>MAPKGTSLDEKKERLLEEMLKRGEIYSNKTIETLSKPTGISSMVIKNVLQALVNEDLVDTDKIGASTYYWCFASKRSQAARTELARLQKALEEQTNFIDKATARIEELKVGREETEERSSLLKEKLALQVKLEEQRGTFRDLLKNDPDVAQKLRNYTDI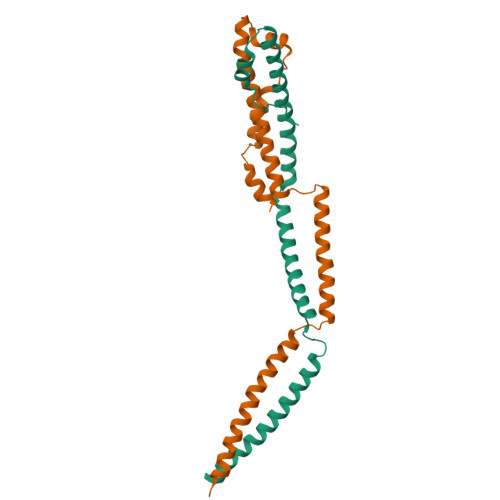AKQEANLWTDNIFCLQKYMLTKLQMDKKTVSTALGITGEFDYLE[3x];>[3x]MAAAYKEAFAAVKELMQTSNKPQNVQTAINNTGSKYGKTTVQKALDELVAQNLCIYTEIGKTGKLYLWNQNLLEVLSDAQLMEVNAQINDLKAQVEKLTQQGETLRITQRNLEAAPITEVLKQEVDELRQQVSANDEKLRLVRESNAIVSDADMLTLQKNYKDAMTAWATRRAKCREVIDTLSEGMGVKPSAFMDQLGLEEGLPMTTYTEMKKALPPVNVSKADIKAALKK>MRTLNFNGKISTLEPLTVTVKNAVSTSGHRLPRNGGFNAAPYFPGTSIRGTLRHAAHKVIVDRVGLNADGKSPFDLAEHFMLAQGVDINGEAETFAPGEINAGAELRSKNPLISLFGRWGLSGKVGIGNAIPDGDNQWGMFGGGARSIMFQRDESLMEFLETDQVDRLERLLEEQAEASVDISQIKTEQDALKKAMKSADKDTKAELQIKVRELDEKIQARKDQKQESRESIRRPIDPYEAFITGAELSHRMSIKNATDEEAGLFISALIRFAAEPRFGGHANHNCGLVEAHWTVTTWKPGELVPVTLGEIVITPNGVEITGDELFAMVKAFNENQSFDFTARGHHHHHH[6x];> MLNFKPYRVIMSSLTPVVISGIAPSLDGILYEALSQAIPSNEPGVVLARLKEILLFNDELGVFHASSLRFGITPEQGIGATTSMRCDYLSPEKLSTAMFSPRTRRGLFTRVLLTGGPTKRRMTTRPAYSAPYLTFDFVGSSEAVEILLNHAHVGVGYDYFSAANGEFNNVTILPLDIDTSISNEGMALRPVPVNSGLNGIKGVSPLIPPYFVGEKLNIVHPAPVRTQLISSLLRG;> MNHPVESVYSALTSILLPYMGEPVPVQRNCSCCGRAPSEFDGVGFELVNAYRERVVHCRPCQTFFVSAPELMGVENPKKPTTGQKFGMWSGVGAVINVEDNSSVLLAPQGVVNKLPEHFFDHVEVITATSGQHLEYLFNTELKFPLIYIQNFGVKTYELVRSLRVSLSADAIYTCADQLLTRQNEVLYMLDLKKAKELHQEIKNYSKKEMDIFIRTVTLLAYSRITPEAASNEFKKNNLIPLLLLLPTDPHQRLSILHLLKKV;> MNTSAVFESAGLSLRKVQQDYIEAAAGALTQDHKVALISAETGVGKTLGYLVPALLILLKNPEAKFVIATNSHALMHQIFRSDRPLLEQIAEQCGIKVTFSRLMGKANYVSLEKVRGLLLMDEFTDLDTVKVLEKLANWSKPLVEFEEEYGELPAQITPEMVTYSIWDDIQDIDDIRLNALSANFIVTTHAMVMVDCMCNHRILGDKENMYLIIDEADIFVDMLEVWKQRRFNLRELTSAFNEHIPRNGVHVIDQLMNDVTSIAGDLHFCSTPAAVALFDNSFNALSKVGREIKNEAARKAFFDCIYSWEMLGLSGGQKGVGVSNKRREPALIAVNPFIGMNVGRYCTQWRSALLTSATLSITSTPETGMEWLCKALGLTSDTISIRKIFSPDVYGSMKLTIAGADFPKVFNDPKEQIFSGQWLKAVVEQLSCIQGPALVLTASHYETRMIANQLGEVSQPVYIQKAGQALSEIIKQYQEKPGILISAGASVGVSPRGENGEQIFQDLIITRIPFLPPDRMKAESLYGYLKERGYSRTFEAVNRNIYLENLRKVIRKAKQSVGRGIRSENDTVRIIILDPRFPEPTDLSSKHRSLEHIIPVRFRREYRSCEILSPAYFEEDIQC

Type IV-A CRISPR-Cas systems diverge from this general mechanism, using a nuclease-independent interference pathway to suppress gene expression for gene regulation and plasmid competition. Here, we present several cryo-EM structures of two evolutionary distant type IV-A1 and type IV-A3 complexes (from Pseudomonas oleovorans and Klebsiella pneumoniae, respectively) bound to cognate DNA targets with and without DinG. The structures reveal multisubunit DNA-surveillance complexes that intimately recognize their DNA-targets to form an R-loop structure. Our results support a model in which DNA-binding is achieved analogously to type I Cascade, while recruitment of DinG differs mechanistically, even in closely related subtypes.

Cryo-EM grid optimization and exhaustive data collection yielded a sufficient amount of particles to reconstruct three structures of the DinG-bound type IV-A3 effector complex, with DinG resolved at ~3 Å to ~7 Å in three distinct states (states I–III). However, density was lacking for the arch domain in state II and only present at low resolution in state III. Similar to the type IV-A1 structure, type IV-A3 DinG is recruited to the NTS at the belly side of the complex. We next compared the three type IV-A3 DinG states, based on a structural alignment of the complexes. This revealed that the Cas8 and Cas5 contacting C-terminus, and Cas7 palm binding segments of α-helices 21 and 22 of DinG, do not rearrange between the states. Thus, the C-terminus and α-helices 21 and 22 appear to anchor DinG to the complex. Between states I and II, the HD domains maintain their relative and overall conformations, while the vFeS moves towards the center of DinG. The arch domain becomes stabilized in state I, as corroborated by the absence and presence of cryo-EM density in states II and I, respectively. Examination of the cryo-EM map also revealed low local resolutions (4–7 Å) for the vFeS domain and NTS exiting the HD2 in all states. This limits the accuracy of structural interpretations and suggests an inherent flexibility within these regions.> VHHPPSYVAHLASDFGVRVFQQVAQASKDRNVVFSPYGVASVLAMLQLTTGGETQQQIQAAMGFKIDDKGMAPALRHLYKELMGPWNKDEISTTDAIFVQRDLKLVQGFMPHFFRLFRSTVKQVDFSEVERARFIINDWVKTHTKGMISHLLGTGAVDQLTRLVLVNALYFNGQWKTPFPDSSTHRRLFHKSDGSTVSVPMMAQTNKFNYTEFTTPDGHYYDILELPYHGDTLSMFIAAPYEKEVPLSALTNILSAQLISHWKGNMTRLPRLLVLPKFSLETEVDLRKPLENLGMTDMFRQFQADFTSLSDQEPLHVALALQKVKIEVNESGTVA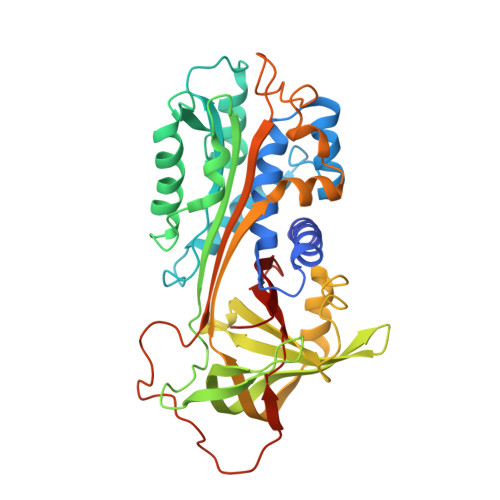SSSTAVIVSARMAPEEIIIDRPFLFVVRHNPTGTVLFMGQVMEP>[4x]MIFMRKVVAEVSIIPLGKGASVS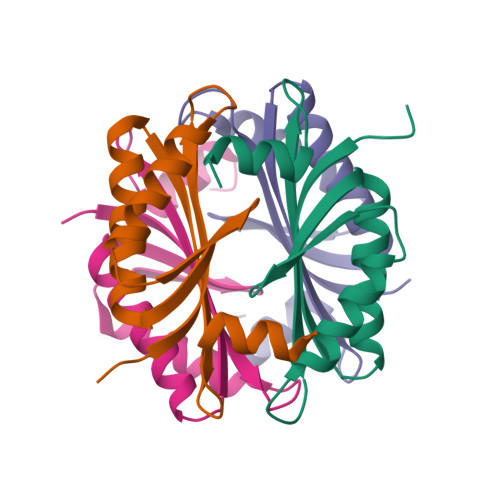KYVKKAIEVFKKYDLKVETNAMGTVLEGDLDEILKAFKEAHSTVLNDVDRVVSSLKIDERKDKENTIERKLKAIGEL> MLPNTKLHNTIFSETRKFTRESFKEIEHLTARLAND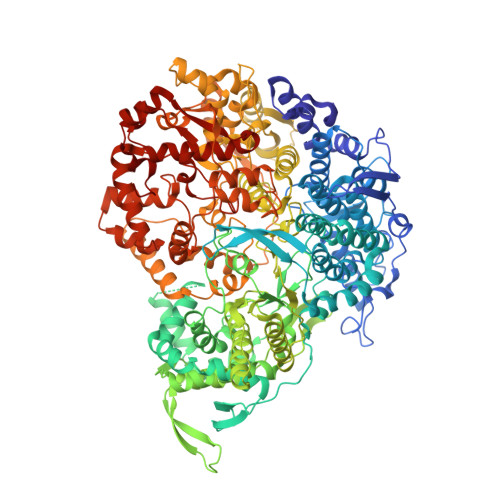RVARHDFLFNTSIVLISDYSGEDSNGNQLQATITIPNEIINPKEYDPSDYPLAEDESFFKQGHKYDYLVTFRAGSLTNTYEPKTKMYKLHAALDKLMHVKQRKSRFADLWRELCAVIASLDVWYQTTNYPLRTYVKLLFHKGDEFPFYESPSQDRIIFNDKSVASILPTFVYTCCQVGTAIMSGILTHVESIVAMNHFLHCAKDSYIDEKLKIKGIGRSWYQEALHNVCQATVPVWSQFNEVIGHRTKSTSEPHFVSSTFISLRAKRAELLYPEFNAYINRAIQLSKTQNDVANYYAACRAMTNDGTFLATLTELSLDAAVFPRIEQHLVTRPAVLMSNTRHESLKQKYTNGVGSIAQSYLSSFTDEIAKRVNGRHHDEAWLNFLTTSSPGRKLTEIEKLEVGGDVAAWSNSRIVMQAVFAREYRTPERIFKSLKAPIKLVERQQSDRRQRAISGLDNDRLFLSFMPYTIGKQIYELNDNAAQGKQAGNAFDIGEMLYWTSQRNVLLSSIDVAGMDASVTTNTKDIYNTFVLDVASKCTVPRFGPYYAKNMEVFEAGNRQSQVRYVNAAWQACALEAANSQTSTSYESEIFGQVKNAEGTYPSGRADTSTHHTVLLQGLVRGNELKRASDGKNSCLATIKILGDDIMEIFQGSESDTYDHAVSNASILNESGFATTAELSQNSIVLLQQLVVNGTFWGFADRISLWTREDTKDIGRLNLAMMELNALIDDLVFRVRRPEGLKMLGFFCGAICLRRFTLSVDNKLYDSTYNNLSKYMTLTKYDKNPDSDSTLMSLILPLAWLFMPRGGEYPAYPFERRDGTFTEDESMFTARGAYKRRLLYDVSNIGEMIQQNSMALDDDLLHEYGFTGALLLIDLNILDLIDEVKKEDISPVKVSELATSLEQLGKLGEREKSRRAASDLKIRGHALSNDIVYGYGLQEKIQKSAMATKETTVQSKRVSSRLHDVIVAKTRDYKISTIPADALHLHEFEVEDVTVDLLPHAKHTSYSSLAYNMSFGSDGWFAFALLGGLDRSANLLRLDVASIRGNYHKFSYDDPVFKQGYKIYKSDATLLNDFFTAISAGPKEQGILLRAFAYYSLYGNVEYHYVLSPRQLFFLSDNPVSAERLVRIPPKYYVSTQCRALYNIFSYLHILRSIANNRGKRLKMVLHPGLIAYVRGTSQGAILPEADNV2-amino-6-[(1S,2R)-2-(3'-methoxybiphenyl-3-yl)cyclopropyl]-3-methylpyrimidin-4(3H)-one 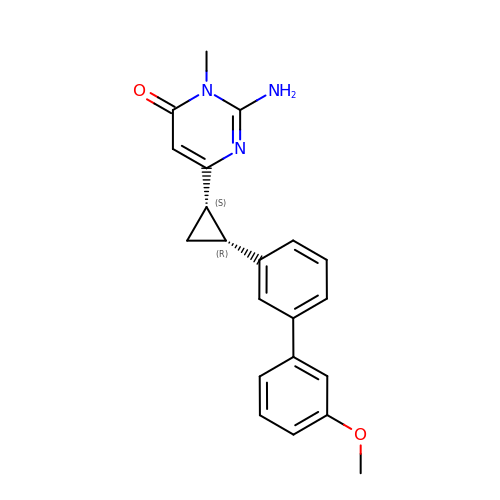| C21 H21 N3 O2 | QECXNBWGUGUPSI-ROUUACIJSA-N> GGMRIEIKLLPLQDNPVIPFNYNYELYSQIVEKAGAIEPRIVKLLESPHGYWTFSRIIIRKREIIPEKGIKILSDDISLYISSSNKEIIKGIVEGIEKSPEFKIGDVGFLVADIKALKSKEIKNVNIFSTLSPIVVRTVKFEGDKLKHWDLYPHDELFLDRLRKVMLLRY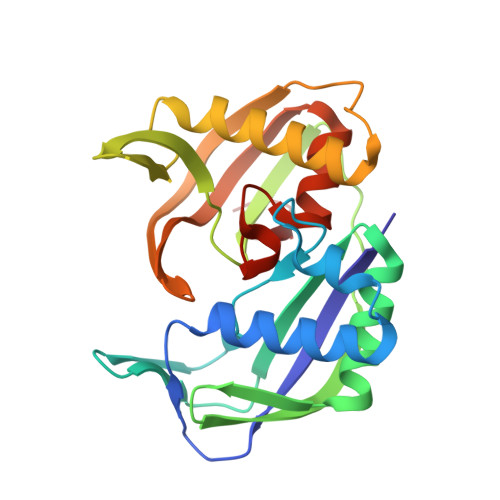HEVMGDLPEDKDFRIELIKFKPTRLIVKDSYIRGSLMVFRYYGSKEIAKFGYENGFGEKTNLGFGMVKIIEEQ>MAPLGPTGPLPQSFLLKCLEQMRKVQADGTALQETLCATHQLCHPEELVLLGHALGIPQPPLSSCSSQALQLMGCLRQLHSGLFLYQGLL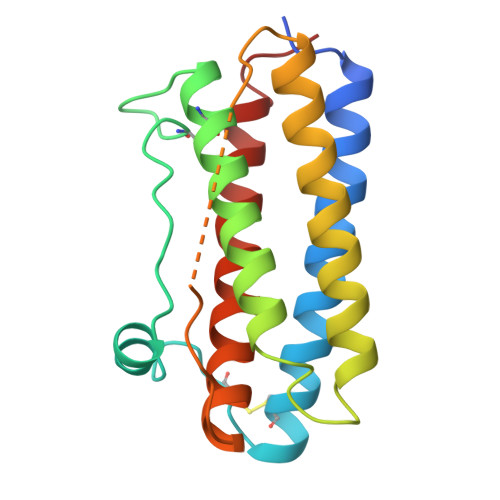QALAGISPELAPTLDTLQLDTTDFAINIWQQMEDLGMAPAVPPTQGTMPAFTSAFQRRAGGVLVASNLQSFLELAYRALRHFAKP[2x]> SVKRLFKVRSDLDFAEQLWCKMSSSVISYQDLVKCFTLIIQSLQRGDIQPWLHSGSNSLLSKLIHQSYHGTMDTVSLSGTIPVQMLLEIGLDKLKKDYISFFIGQELASLNHLEYFIAPSVDIQEQVYRVQKLHHILE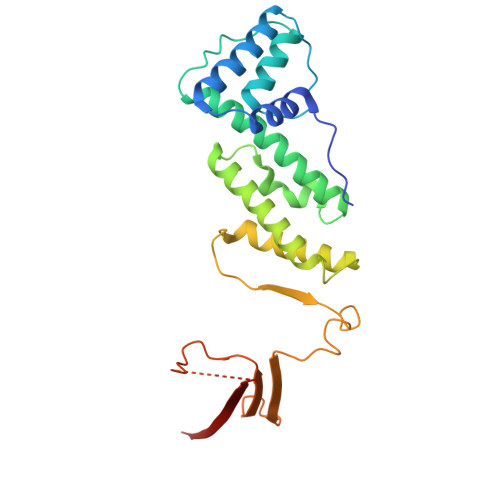ILVSCMPFIKSQHELLFSLTQICIKYYKQNPLDEQHIFQLPVRPTAVKNLYQSEKPQKWRVEIYSGQKKIKTVWQLSDSSPIDHLNFHKPDFSELTLNGSLEERIFFTNMVTCSQVHFK>[2x]MDPNSLMTNRLVLSGTVCRAPLRKVSPSGIPHCQFVLEHRSVQEEAGFHRQAWCQMPVIVSGHENQ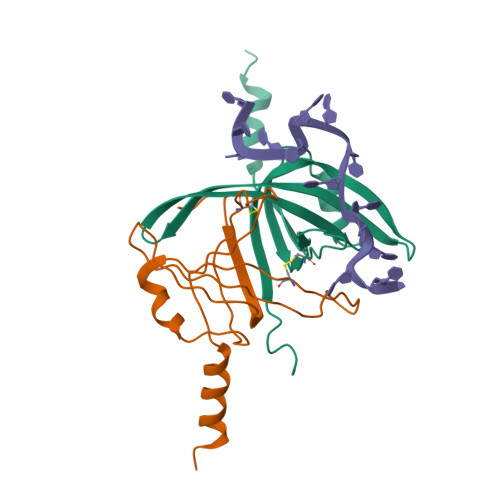AITHSITVGSRITVQGFISCHKAKNGLSKMVLHAEQIELIDSVDKLAAALEHHHHHH>[4x]GSMTDGDYDYLIKLLALGDSGVG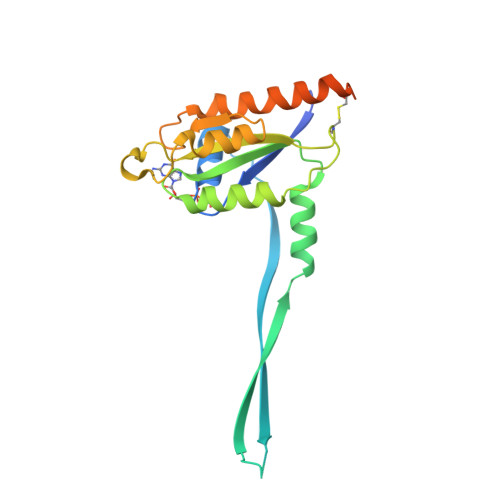KTTFLYRYTDNKFNPKFITTVGIDFREKRVVYDTQGADGASGKAFKVHLQLWDTAGLERFRSLTTAFFRDAMGFLLMFDLTSQQSFLNVRNWMSQLQANAYCENPDIVLIGNKADLPDQREVNERQARELAEKYGIPYFETSAATGQNVEKSVETLLDLIMKRMEKCVEKTQVPDTVNGGNSGKLDGEKPAEKKCAC In this study, we have addressed these questions by focusing on the two PLP-dependent enzymes alanine racemase (ALR) and cystathionine β-lyase (CBL). E. coli CBL is a homotetramer that catalyzes the formation of l-homocysteine from l-cystathionine. We have demonstrated that two non-homologous specialized enzymes from E. coli are as little as one mutation away from being physiologically relevant replacements for each other.

The inhibitor, (R)-1-aminoethylphosphonic acid (l-Ala-P), is a phosphonate analogue of l-Ala that is a substrate for the transaldimination reaction, in which the Schiff base linkage between Lys-34 and PLP in the active site of the resting enzyme is displaced by the amino group of the incoming substrate. Thus, l-Ala-P forms a stable external aldimine with PLP in the ALR active site. Binding of l-Ala-P to ALR(Y274F) did not induce any significant conformational changes in the dimer (root-mean-square deviation = 0.16 Å over 715 Cα atoms), although we also note that the ligand-bound structure was generated by soaking. Formation of the external aldimine tilts the plane of the PLP pyridine ring by ∼10° toward Tyr-255′. Tyr-255′ is positioned to act as the catalytic base, with a distance of 3.3 Å from its side chain hydroxyl group to Cα of the substrate. The side chain amino group of the catalytic acid, Lys-34, is 4.1 Å from Cα. There was clear electron density for the l-isomer but not the d-isomer of the inhibitor, confirming that there had been no observable racemization of l-Ala-P. The orientation of l-Ala-P in the active site of our ALR structure illuminates the role of the Y274F mutation in enhancing CBL activity. To test this hypothesis, a cystathionine-PLP adduct was built and docked into the active site of ALR(Y274F) using GOLD. In this docked model, the Cα atoms of l-Ala-P and cystathionine overlay, and the distal carboxylate of cystathionine is perfectly positioned to engage in a salt bridge with the side chain of Arg-280′.

>MQAATVVINRRALRHNLQRLRELAPASKMVAVVKANAYGHGLLETARTLPDADAFGVARLEEALRLRAGGITKPVLLLEGFFDARDLPTISAQHFHTAVHNEEQLAALEEASLDEPVTVWMKLDTGMHRLGVRPEQAEAFYHRLTQCKNVRQPVNIVSHFARADEPKCGATEKQLAIFNTFCEGKPGQRSIAASGGILLWPQSHFDWVRPGIILYGVSPLEDRSTGADFGCQPVMSLTSSLIAVREHKAGEPVGYGGTWVSERDTRLGVVAMGFGDGYPRAAPSGTPVLVNGREVPIVGRVAMDMICVDLGPQAQDKAGDPVILWGEGLPVERIAEMTKVSAYELITRLTSRVAMKYVD[4x]> GPLGSHMHRQPPEYNPNDEEEEEVQLKSARRATSMDLPMPMRFRHLKKTSKEAVGVYRSPIHGRGLFCKRNIDAGEMVIEYAGNVIRSIQTDKREKYYDSKGIGCYMFRIDDSEVVDATMHG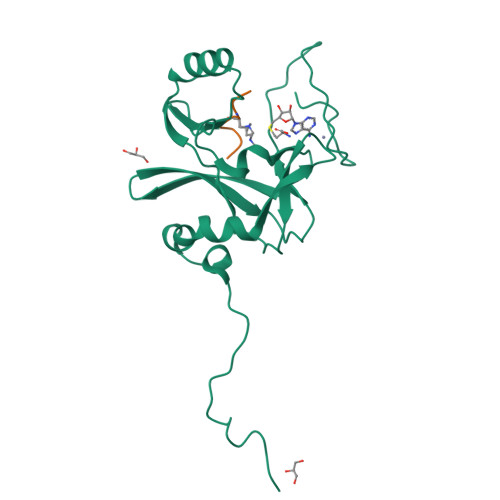NAARFINHSCEPNCYSRVINIDGQKHIVIFAMRKIYRGEELTYDYKFPIEDASNKLPCNCGAKKCRKFLN;> ARTKQTARY>MAYVPLSGTNVRILADVPFSNDYKNTRWFTSSS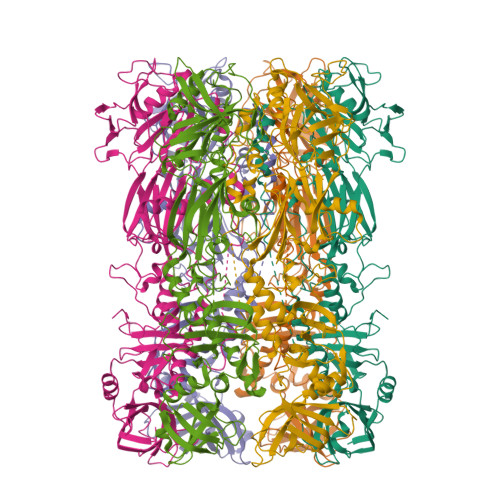NQYNWFNSKSRVYEMSKVTFMGFRENKPYVSVSLPIDKLYSASYIMFQNADYGNKWFYAFVTELEFKNSAVTYVHFEIDVLQTWMFDIKFQESFIVREHVKLWNDDGTPTINTIDEGLSYGSEYDIVSVENHKPYDDMMFLVIISKSIMHGTPGEEESRLNDINASLNGMPQPLCYYIHPFYKDGKVPKTYIGDNNANLSPIVNMLTNIFSQKSAVNDIVNMYVTDYIGLKLDYKNGDKELKLDKDMFEQAGIADDKHGNVDTIFVKKIPDYEALEIDTGDKWGGFTKDQESKLMMYPYCVTEITDFKGNHMNLKTEYINNSKLKIQVRGSLGVSNKVAYSVQDYNADSALSGGNRLTASLDSSLINNNPNDIAILNDYLSAYLQGNKNSLENQKSSILFNGIMGMIGGGISAGASAAGGSALGMASSVTGMTSTAGNAVLQMQAMQAKQADIANIPPQLTKMGGNTAFDYGNGYRGVYVIKKQLKAEYRRSLSSFFHKYGYKINRVKKPNLRTRKAFNYVQTKDCFISGDINNNDLQEIRTIFDNGITLWHTDNIGNYSVENELRHHHHHH[2x]>[4x]MIISTLETNLIWQAALRAVQAASDHAS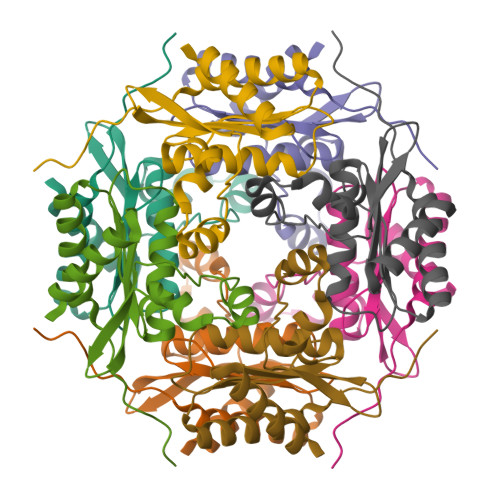ALGIRIHVAVVDRAGLNLVFLSMNGAFLHSADIARDKAYTAAGFGFPTGQWLQVLGDNERLRIGIPARERLVVFGGGLPVLLDRQCIGGIGVSGGSEEQDEACAEAGLRAMLG>GSTSPVAQWEFHPGHFWMRGKRPDKIVDYDEELQLWNVYGYPESAAILSNPKVFSSDTMRLDPIKLDEAIVEGDFAHTDPPKHRRLRGLVDHAFTPSLVAKMESRVHGIIHELLDGVEGKSQFDLVAEFAAPLPLIMISDLLGVPESDRALFRQWMDKMLDGSEKFESPETVLEQEEELHKELELLWEMRDYWHERAAESRKRPREDLISQLVHAEVDGQKLNDSQISNIANRLLVNGHLTTAMLIANTMLCLDAFSDQDARVRADRSLVPALLEESMRYMSPICGVGRATNSEVEVAGT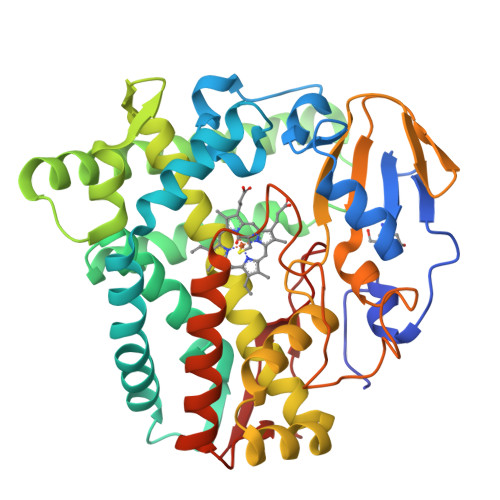VIPKDQLLLVWTGAANRDERQFEKPDVFDAGRSPNAHLGLGRGIHFCLGRQLARMESKAAVEILLDRLPTLRADPANPPTFLQVVDASGVATLPVVTQ[4x]(S)-2-(2-(6-amino-9H-purin-9-yl)ethoxy)-3-phosphonopropanoic acid | C10 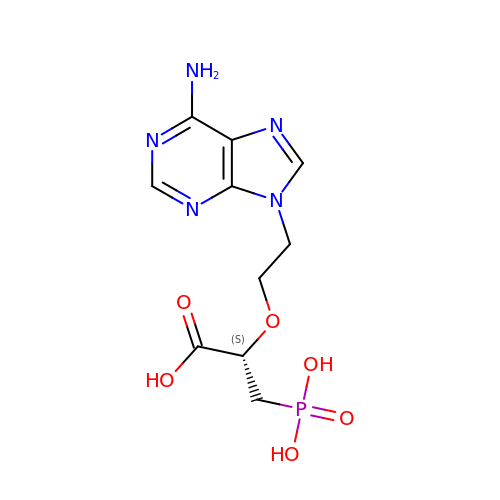H14 N5 O6 P | AGUNSWPLTCYYSO-ZCFIWIBFSA-N> GMHHQRKTHVDNNIAAVELAKAYRLLNHGPTVLVSARSQGIDNVMAAAWCCALDFAPPKLTVVLDKMTKTREFIEQSGMFVIQVPTVAQLQLTHRVGSQSLADDANKLLNCGVELFEMAGHDLPFVAGCSAWLACKLIPEPN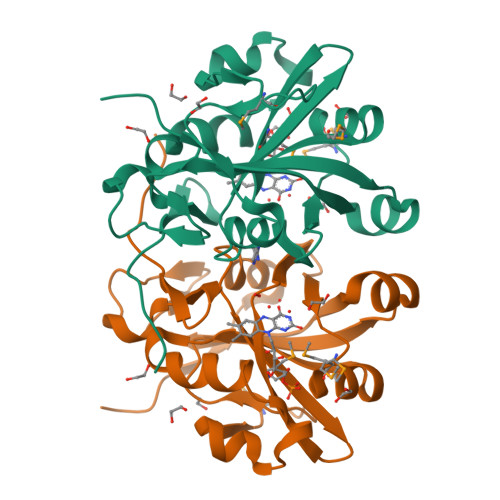NQLQYDLFIAEVIGAWADTQVFNHGHWHFDTAPADKRSLHYIAGGQFYAIGESFNAD>MTSKIEQPRWASKDSAAGAASTPDEKIVLEFMDALTSNDAAKLIEYFAEDTMYQNMPLPPAYGRDAVEQTLAGL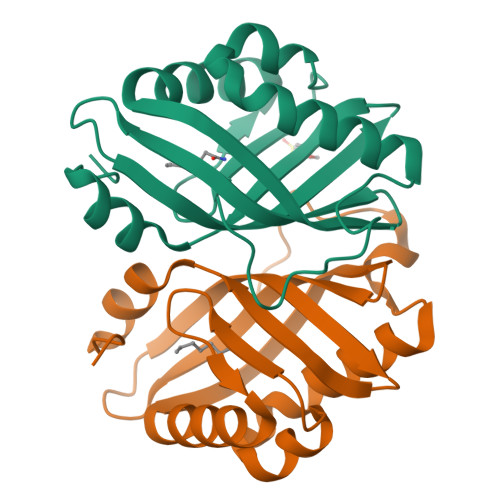FTVMSIDAVETFHIGSSNGLVYTERVDVLRALPTGKSYNLSILGVFQLTEGKITGWRDYFDLREFEEAVDLPLRG[2x]Here, we report the discovery and identification of a novel lipase from Lasiodiplodia theobromae fungus (LTL1), which hydrolyses C8–C10 ME efficiently. LTL1 can perform hydrolysis over pH ranges from 3.0 to 9.0 and maintain thermotolerance up to 70 °C. It has high selectivity for monoesters over triesters and displays higher activity over commercially available lipases for C8–C10 ME to achieve 96.17% hydrolysis within 31 h. To obtain a steady source of C8 and C10 fatty acids, hydrolysis of C8-C10 ME can be carried out enzymatically with lipases and esterases. These enzymes catalyse the hydrolysis of ester bonds of tri-, di-, and monoglycerides into fatty acids and alcohol. Structural analysis by protein X-ray crystallography revealed LTL1’s well-conserved lipase core domain, together with a partially resolved N-terminal subdomain and an inserted loop, which may suggest its hydrolytic preference for monoesters.

To gain further insights into its selectivity for monoesters over triesters, we solved the 3D structure of LTL1 by protein X-ray crystallography. The crystal structure of LTL1 consists of two nearly identical polypeptide chains covering amino acid residues 83-449 (chain A) and 84-449 (chain B) of L. theobromae lipase B (UniprotKB: A0A5N5DNA6), respectively. These residues fold into lipase core domains (yellow and cyan) with N-terminal extensions (orange and pink) and inserted loops (magenta and blue) and are in close contact with each other through an extensive interfacial area of 1229 Å2 according to PISA analysis. The N-terminal portion of the expressed LTL1 (residues 19–82) could not be resolved in the structure, likely due to proteolysis during crystallisation. The model predicts that LTL1 has an N-terminal subdomain residing above the active site, which seems to be plausible given its accurate reconstruction of the core domain and correct prediction of the secondary structure (i.e., the two alpha helices, coloured orange in the X-ray structure and dark green in the model) of the N-terminal extension observed in the crystal structure. When compared with CALB, both LTL1 and AFLB have an extra N-terminal subdomain, albeit with a different size and conformation, and an inserted loop flanked by two cysteines that form a disulphide bond. The loop in AFLB flips inwards, covering the active site, whereas the loop in LTL1 bends outwards, leaving LTL1 in an “open state” that has similarly been observed in CALB. With the help of the intact N-terminal subdomain, LTL1’s loop could potentially reorientate and at least partially cover the active site, as predicted by the AlphaFold2 model. The presence of the additional N-terminal subdomain and inserted loop covering the active site seems to suggest that steric effects could be part of the reason for LTL1’s preference for slimmer monoesters over bulkier triesters.

>APAPVPENGLEKRQSLSSVLSALSGLTEPTAILSQLEAVEATSTPTSVEQAQEQLEAIYGTTPTNIFENIAQQIADGLSTLTIVQALGFSPSGENSETNSNTREPSTTIYPKKSSSDAPYSITEEELRQAIYIPSDFTYGDKPPVIFVPGTGSYGGISFGSNLRKLLTGVSYADPVWLNVPDALLRDAQTNGEFVAYAINYISGISGDANVSVVSWSQGGLDTQWAFTYWPSTRALVSDFVPVSPDFHGTVLANVICLNPGAGGVGLGPCAPAVLQQEYNSNFVTALRAAGGADAYVPTTSVFSGFLDEIVQPQSGTGASAYINDARGVGTTNAEVQVVCKGKGPAGGFYTHESLLVNPLTYALLVDALTHDGPGSVDRLDLDTVCSTVVAPGLGLDALLEIEGVNVLAAVNLLTYSDRRLAEPALMSYAA[2x]N-[2-(5-methoxy-1H-indol-3-yl)ethyl]-2,2-dimethylpropanamide | C16 H22 N2 O2 | 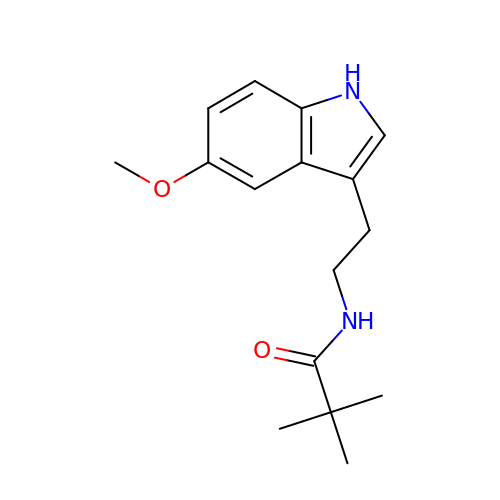CUMVZJLZCUYFCZ-UHFFFAOYSA-N>[8x]MIRNGFYIIKDRFFSDMSDPYLKGNKKQNRPHYYCFEDSNYNGIYWMIPLSSRIDKYKKIVSKRTG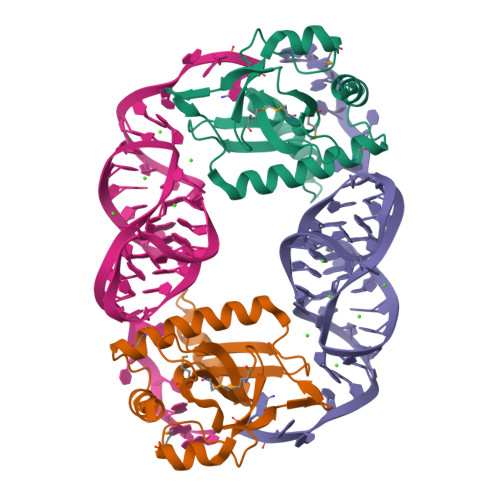KGRNCDIIHIVKLDDSHESAFLIQDMFPISDKYIEREYTIAGNHLRLTSEHAAKEIEQKARKVLGMLKRGIKFTPTQPDIQKIYERLQQ> MASVSSATFSGHGARSLLQFLRLVGQLKRVPRTGWV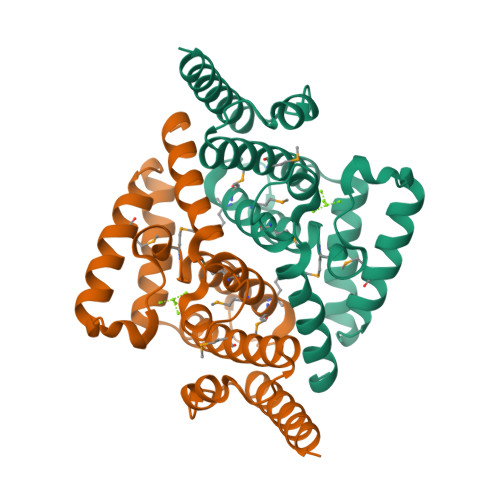YRNVQRPESVSDHMYRMAVMAMVIKDDRLNKDRCVRLALVADMAECIVGDIAPADNIPKEEKHRREEEAMKQITQLLPEDLRKELYELWEEYETQSSAEAKFVKQLDQCEMILQASEYEDLEHKPGRLQDFYDSTAGKFNHPEIVQLVSELEAERSTNIAAAASEPHS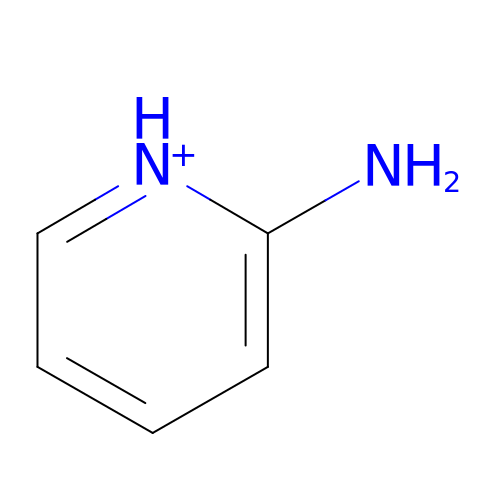2-AMINOPYRIDINE | C5 H7 N2 | ICSNLGPSRYBMBD-UHFFFAOYSA-O>MSKIRIGIVGYGNLGRGVEAAIQQNPDMELVAVFTRRDPKTVAVKSNVKVLHVDDAQSYKDEIDVMILCGGSATDLPEQGPYFAQYFNTIDSFDTHARIPDYFDAVNAAAEQSGKVAIISVGWDPGLFSLNRLLGEVVLPVGNTYTFWGKGVSQGHSDAIRRIQGVKNAVQYTIPIDEAVNRVRSGENPELSTREKHARECFVVLEEGADPAKVEHEIKTMPNYFDEYDTTVHFISEEELKQNHSGMPHGGFVIRSGKSDEGHKQIIEFSLNLE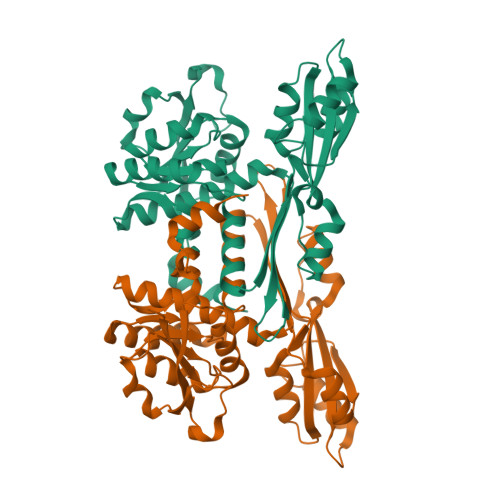SNPMFTSSALVAYARAAYRLSQNGDKGAKTVFDIPFGLLSPKSPEDLRKELLTRHHHHHH[2x]>[3x]PMFIVNTNVPRASVP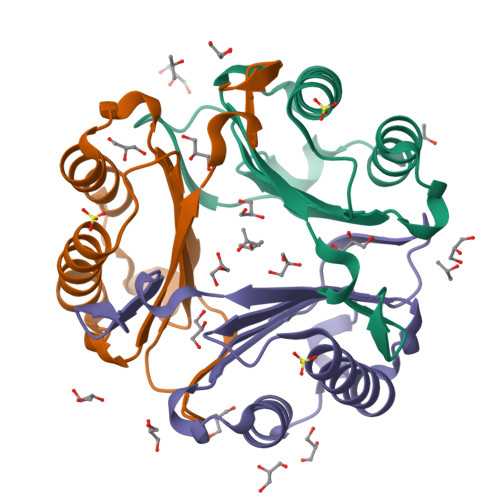DGFLSELTQQLAQATGKPPQYIAVHVVPDQLMAFGGSSEPCALCSLHSIGKIGGAQNRSYSKLLCGLLAERLRISPDRVYINYCDMNAANVGWNNSTFA> MRGSHHHHHHGSMEQSHQNLQSQFFIEHILQILPHRYPMLLVDRITELQANQKIVAYKNITFNEDVFNGHFPNKPIFPGVLIVEGMAQSGGFLAFTSLWGFDPEIAKTKIVYFMTIDKVKFRIPVTPGDRLEYHLEVLKHKGMIWQVGGTAQVDGKVVAEAELKAMI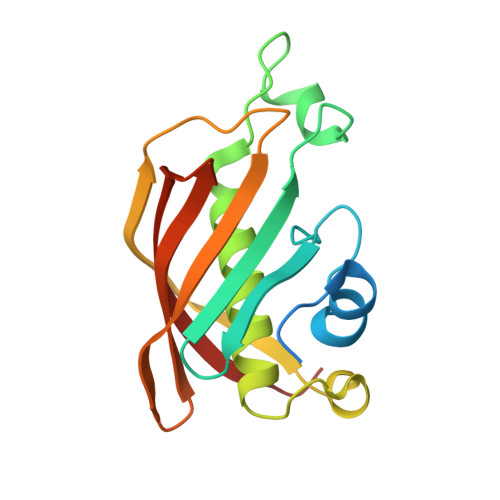AERE Previously, BLEG-1 (formerly termed Bleg1_2437 and Bleg1_2478) from Bacillus lehensis G1 was identified as a member of the metallo-hydrolase-like MBL-fold superfamily which exhibited enzymatic activity and predicted structural characteristics similar to the B3 subclass metallo-β-lactamase (MBL) antibiotics-degrading enzyme (E.C. 3.5.2.6). MBLs degrade β-lactam antibiotics by breaking the four-membered β-lactam ring, destructing their core structure and deactivating the antibacterial properties, thus conferring antimicrobial resistance to bacteria. On the other hand, GLXII (E.C. 3.1.2.6) is one of the key enzymes in the glyoxalase system involved in the detoxification of methylglyoxal, a cytotoxic product of glycolysis and other metabolic activities by converting S-D-lactoylglutathione (SLG) to produce non-toxic D-lactate in the presence of glutathione (GSH).

The crystal structure of BLEG-1 solved at 1.44 Å resolution unveiled structural features which may have contributed to its promiscuity and evolutionary divergence. Diffraction of BLEG-1 single protein crystal showed that it has a space group of P41212 with one molecule in each asymmetric unit, completeness of 98% and Rmerge of 0.045. Solved 3D structure of BLEG-1 showed a global topology of an αβ/βα sandwich fold, with the active binuclear center located at the interface of N and C-terminal domain. At the binuclear center, both zinc ions are coordinated via trigonal bipyramidal geometry in which Zn1 is coordinated by His-54, His-56, and His-131 residues, while Zn2 is coordinated by Asp-58, His-59, and His-191 residues. The zinc ions are separated by a distance of 3.3 Å and are bridged by Asp-150 residue and a water molecule, Wat1. Another water molecule, Wat2, is interacting with Zn2 at the apical or axial position. Analyses on the global structure of BLEG-1, L1 B3 MBL, YcbL and GloB GLXIIs revealed that the enzyme showed higher resemblance to GLXII, particularly to YcbL, a GLXII-2. Yet, the active site architecture of BLEG-1 resembled that of L1 B3 MBL, which allowed the accommodation of β-lactam other than SLG. The insertion of active-site loop in the N-terminal domain of BLEG-1 active site formed a configuration similar to B3 MBL binding cavity which eventually allowed the accommodation of β-lactams. We propose that BLEG-1 could possibly have evolved from GLXII and adopted MBL activity through this insertion.

> MFKQIPLGPIQTNAYVLYNDDKEAVIFDPGGDAEALITWLKREQLTPLAILLTHAHFDHIGAVDAVRDTFSIPVYLHTKERHWLEDPALNGSSRLTGRPITTAKPADHLLTNEKSLTIGTFTFSVFHTPGHSPGSVSYYYQKEAVLFSGDVLFQQSIGRTDLRGGDHTLLLASIHNKILPLPERTIVASGHGPLTTIGQEMDHNPFLTGY> QLTPTFYDNSCPNVSNIVRDTIVNELRSDPRIAASILSLHFEDCFVNGCDASILLDNTTSFRTEKDAFGNANSARGFPVIDRMKAAVESACPRTVSCADLLTIAAQQSVTLAGGPSWRVPLGRRDSLQAFLDLANANLPAPFFTLPQLKDSFRNVGLNRSSDLVALSGGHTFGKNQCRFIMDRLYNFSNTGLPDPTLNTTYLQTLRGLCPLNGNLSALVDFDLRTPTIFDNKYYVNLEEQKGLIQSDQELFSSPNATDTIPLVRSFANSTQTFFNAFVE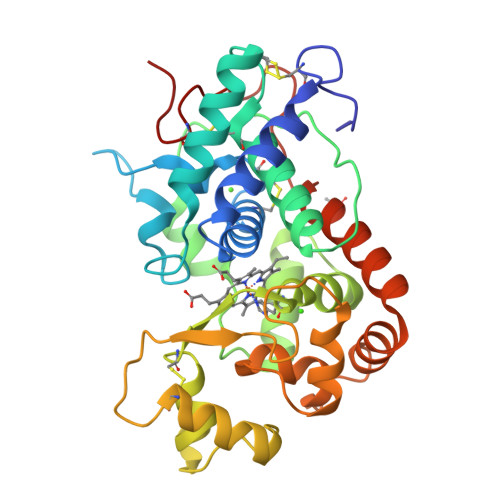AMDRMGNITPLTGTQGQIRLNCRVVNSNS>[4x]GILTIRLLMHGKEVGSIIGKKGESVKRIREESGARINISEGNCPERIITLTGPTN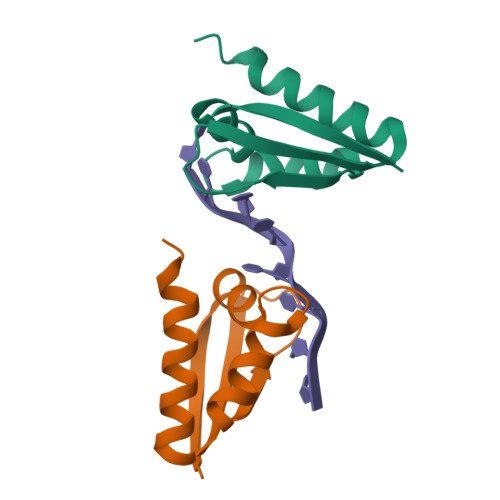AIFKAFAMIIDKLEEDINS4-methylsulfanyl-~{N}-(4-pyridin-2-yl-1,3-thiazol-2-yl)benzamide | C16 H13 N3 O S2 | 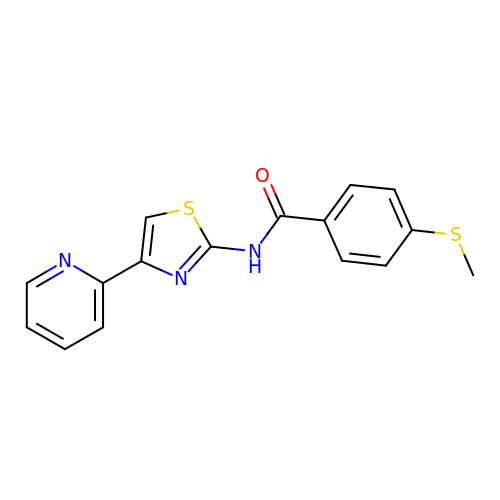NZGXQIAKLVEMPP-UHFFFAOYSA-N>[3x]MDFRIGEGYDVHQLVPGRPLIIGGVTIPYERGLLGHSDADVLLHAITDALFGAAALGDIGRHFSDTDPRFKGADSRALLRECASRV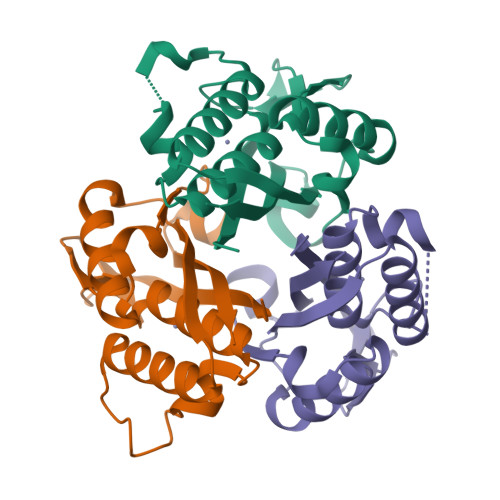AQAGFAIRNVDSTIIAQAPKLAPHIDAMRANIAADLDLPLDRVNVKAKTNEKLGYLGRGEGIEAEAAALVVR>GSLPVASVSLDTVTVSPSAPYTDTNGLLTDYGNASASPWMKKLQSVAQGSGETFRILQIGDSHTAGDFFTDSLRKRLQKTWGDGGIGWVYPANVKGQRMAAVRHNGNWQSLTSRNNTGDFPLGGILAHTGSGGSMTLTASDGIASKQRVSLFAKPLLAEQTLTVNGNTVSANGGGWQVLDTGAALPLTIHTEMPWDIGFINIENPAGGITVSAMGINGAQLTQWSKWRADRMNDLAQTGADLVILSYGTNEAFNNNIDIADTEQKWLDTVRQIRDSLPAAGILIIGAPESLKNTLGVCGTRPVRLTEVQQMQRRVARQGQTMFWSWQNAMGGICSMKNWLNQGWAAKDGVHFSAKGYRR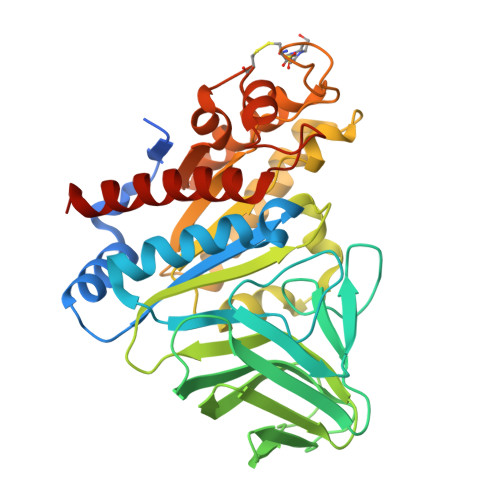AAEMLADSLEELVRSAAIRQ[2x]>MAKTVETVLGPVPVEQLGKTLIHEHFLFGYPGFQGDVTRGTFREDEALRVAVEAAEKMKRHGIQTVVDPTPNDCGRNPAFLRRVAEETGLNIICATGYYYEGEGAPPYFQFRRLLGTAEDDIYDMFMAELTEGIADTGIKAGVIKLASSKGRITEYEKMFFRAAARAQKETGAVIITHTQEGTMGPEQAAYLLEHGADPKKIVIGHMCGNTDPDYHRKTLAYGVYIAFDRFGIQGMVGAPTDEERVRTLLALLRDGYEKQIMLSHDTVNVWLGRPFT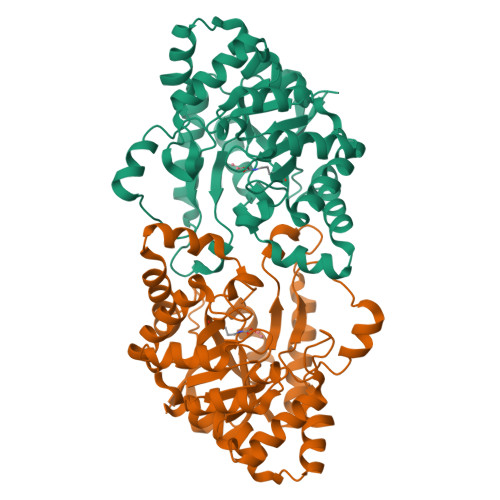LPEPFAEMMKNWHVEHLFVNIIPALKNEGIRDEVLEQMFIGNPAALFSAHHHHHH[2x]> AFTGVERSTIGAIAKILASTPE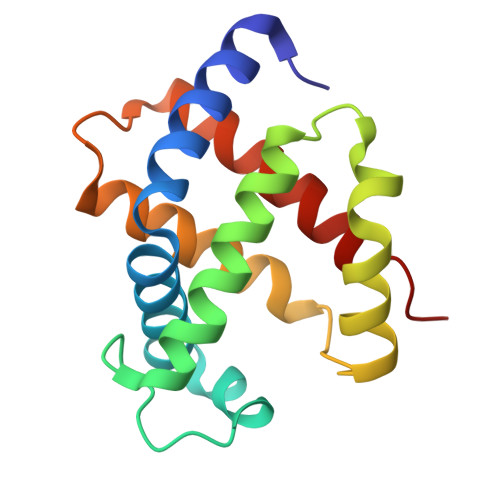AYGAEALARLFATHPGAKSYFDYADYSAAGAKVQLHGGKVIRAVVSAAEHDDDLHAHLMVLAVTHGKKLLVDPSNFPMLSECILVTLATHLAEFSPATHCAVDKLLSAISSELSSKYR> THYSNIEANESEEVRQFRRLFAQLAGDDMEVSATELMNILNKVVTRHPDLKTDGFGIDTCRSMVAVMDSDTTGKLGFEEFKYLWNNIKRWQAIYKQFDTDRSGTICSSELPGAFEAAGFHLNEHLYNMIIRRYSDESGNMDFDNFISCLVRLDAM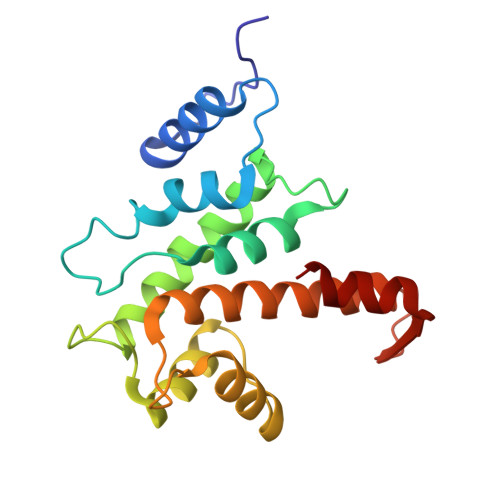FRAFKSLDKDGTGQIQVNIQEWLQLTMYS>SNAMIRCAKKEDLNAILAIYNDAIINTTAVYTYKPQTIDERIAWFETKQRNHEPIFVFEENGSVLGFATFGSFRPWPAYQYTIEHSIYVDASARGKGIASQLLQRLIVEAKAKGYRTLVAGIDASNEASIKLHQKFNFKHAGTLTNVGYKFDYWLDLAFYELDLKD[2x]

The Gcn5-related N-acetyltransferases (GNATs) are a very large enzyme superfamily with more than 10,000 members identified across all kingdoms of life. The GNATs catalyse the transfer of an acetyl group from acetyl CoA to the primary amine of substrates including antibiotics aminoglycosides, glucosamine-6-phosphate, histones, serotonin, spermine, spermidine, and other small molecules. Members of the family share a common fold known as the GNAT fold, comprised of 6–7 anti-parallel β-strands and 4 α-helices in the topology β1-α1-α2-β2-β3-β4-α3-β5-α4-β6-β7. Staphylococcus aureus, an important pathogenic and increasingly multi-drug resistant bacterium, contains 35 putative GNAT enzymes, many of which remain uncharacterised both functionally and structurally.

Here, we describe the 2.15 Å structure of a GNAT family member within S. aureus. SaGNAT protein crystals produced in 1 M sodium acetate trihydrate, 100 mM HEPES pH 7.5, and 50 mM cadmium sulphate diffracted to 2.15 Å and were indexed and integrated in the space group C2, with unit cell parameters a = 97.5 Å, b = 78.9 Å, c = 66.0 Å, α = 90°, β = 112.0°, γ = 90°. The refined x-ray crystallographic structure revealed SaGNAT to be an α/β protein comprised of 4 α-helices and 7 β-strands, with a topology β1-α1-α2-β2-β3-β4-α3-β5-α4-β6-β7. Two central antiparallel β-sheets (β1–4 and β5–8) are splayed between β4 and β5 to create a V-shape in the protein. The two β-sheets are held together at the V joint by hydrogen bonding located on the N-terminal residues in strands β4–β5, and diverge at Ser83 and Ala117. This signature feature of GNATs is stabilised by hydrogen bond interactions between water molecules and the amide N and carbonyl O atoms from the protein main chain. SaGNAT is likely to exist as a dimer based on the crystal structure, structural similarity with homologous proteins, and elution profiles from size exclusion chromatography. In the asymmetric unit of the crystal, two SaGNAT molecules were present with a buried surface area of 1,397 Å2, strongly suggesting that this interaction is biologically relevant. Briefly, the binding interface in comprised Ala75:Tyr28/Tyr146; Tyr30:Gln77; Arg71:Glu81; Thr140:Ala138; Thr114:Thr142/Asn143; Thr79:Val144; Thr142:Glu158; Asp160:Asn143. The structure confirms that the protein exhibits the core GNAT fold, and has high structural homology with phosphinothricin acetyltransferases.> HHHHHHMPSGGVFSGSVNLKHVKLGYQYLVNHFLTLLLVPVMAATALELARLGPGELLSLWRSLELDLVHILCSAFLVVFVGTVYVMSRPRPVYLVDYACYKPPASCRVPFATFMEHTRLISDDDKSVRFQTRILERSGLGEDTCLPPANHYIPPNPSMEASRAEAQLVIFSAIDD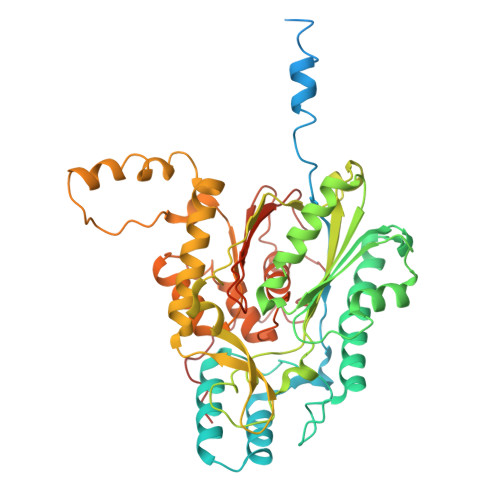LVRRTGLKPKDIDILVVNCSLFSPTPSLSAMIINKYKLRSNIRSFNLSGMGCSAGLISIDLARDMLQVHPNSNALVVSTEIITPNFYQGSRRDMLLPNCLFRMGAAAILLSNRRREARRAKYRLVHVVRTHKGADDRAYRCVYEEEDEQGFSGISLSKELMAIAGDALKSNITTIGPLVLPMSEQLLFFFRLVGRKLVNKGWRPYIPDFKLAFEHFCIHAGGRAVIDELQKNLQLSPRHVEASRMTLHRFGNTSSSSLWYELAYIEAKGRMRRGDRVWQIGFGSGFKCNSAVWKCLRSIKTPTNGPWDDCIHRYPVDVPEVVKL> MVTQLKSASEYDSAL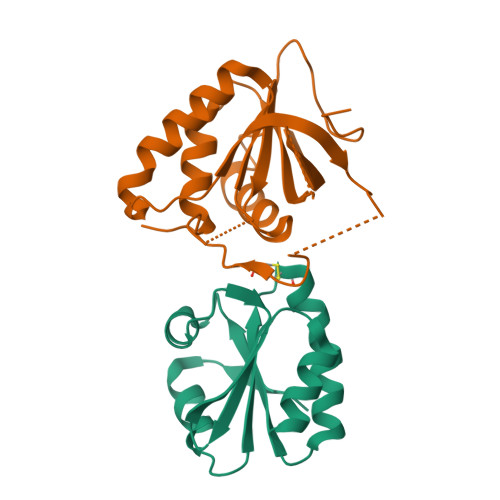ASGDKLVVVDFFATWCGPSKMIAPMIEKFAEQYSDAAFYKLDVDEVSDVAQKAEVSSMPTLIFYKGGKEVTRVVGANPAAIKQAIASNV;> SSLISKTIKYDPAKDKLITLASGSFWGTEHMYRKYLNDRIVDSKVGYANGEESKKDSPSSVSYKRVSGGDTDFAEVLQVSYNPKVITLRELTDFFFRIHDPTTSNSQGPDKGTQYRSGLFAHSDADLKELAKIKEEWQPKWGNKIATVIEPIKNFYDAEEYHQLYLDKNPQGYACPTHYLREM>MESLSEVSVQFSQLSMFPFFDMAHYLASVMSAREQAGALDIASHSPMASWFSAMLHCFGGGILSSILLAEPPVGILANTTNIMLASAIWYMVYYFPYDLFYNCFFFLPIRLIAAGMKEVTRTWKILSGITHAHSHYKDAWLVMITIGWARG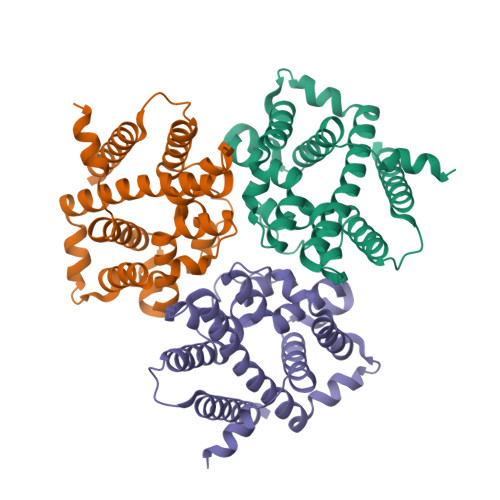AGGGLISNFEQLVRGVWKPESNEFLKMSYPVKVTLIGAVLFTLQHGHYLPISRHNLMFIYTMFLVSIKVTMMLTHSAGSPFLPLETPLHRILFGLRQNQAEVRESPSSSGAKGKPSKKTLDKDSGEQSNKKDKAAAENLYFQGLEDYKDDDDKHHHHHHHHHH[4x]>[2x]MTQVAEIKSPHEQRLEDNIAGKEDIYRESHKRVFKLLERFDGQKPAIDVERALYFTQSMAETVGQPLVLRWAKALMNVAKNITVMVQDDQLLLGRCGGHDGRYGILYPELDGDFLDIAVRDLPTRPQSPASISPEDAKIVVEQIAPFWKGRTYHEALNKALPAEVHKLTYDDPDGLISRFIVNETSSFRSSIQWVHDYEVVLKRGFNGLKQEMEEKLAALDPASPVDQVDKRPFIEATILVCDAIVLWAKRHADAARKAAEACADPVRKAELIRMAENAEHVPANPARDFYEAVQSQYFTQMFSRLEQKTGTTISNGRMDQYFYPFYKKDMEAGILTDEKTLEYLECMWVGMAEFIDMYISPAGGAFNEGYAHWEAVTIGGQTPDGRDATNDLTYLFLKSKREFPLHYPDLAARIHSRAPERYLWDVAE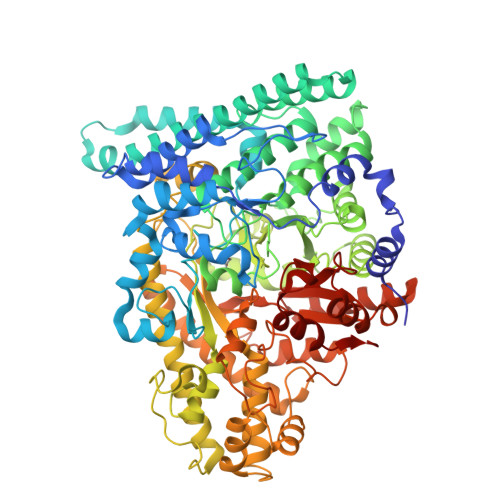TIKFGSGFPKLCNDEECIPLYVSKGATFEEALDYAVSGCIEIRMPNRDTYTSGGAYTNFASAVEMALYDGKMKKYGDVQLGIQTGDARKFKSWDEFWNAYVQQHMLLLRTTFIQQYIVIQTRAKHFAQPMGSVLHALCRKHCIDLHQPQIPEGLNFGYFEFMGLGTVIDSLAAIKKLVFEDKKLTMDQLIDALEANFEGYEDIQQLLRTAPCYGNDDEYADEIGRELDRMAVSFAAKYGKEMGINNDARYVPFTSHVPFGKVVSATPNGRVAWFPLADGSSPSHGADHNGPTAILLSNHNTKNYGMRARAARLINVKFTPKCVEGDAGTEKLVQFIRTWCDLKLWHIQFNVINADTLKKAQKDPQKYRNLIVRIAGYSAYFVDLTPDLQNDLIARTGHDQM ALANINE BORONIC ACID | C2 H8 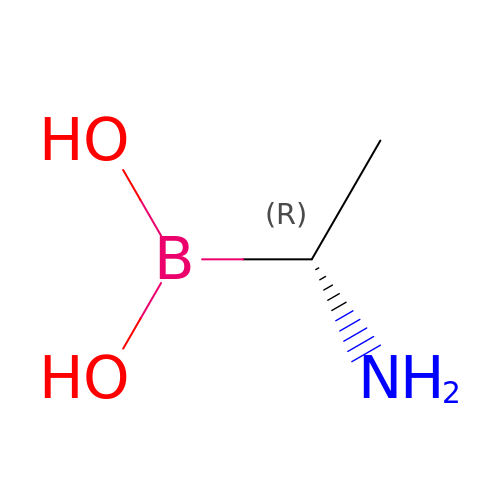B N O2 | MEJXSZPJYPOEIL-REOHCLBHSA-N> TGFNLSIDTVEGNPGSSVVVPVKLSGISKNGISTADFTVTYDATKLEYISGDAGSIVTNPGVNFGI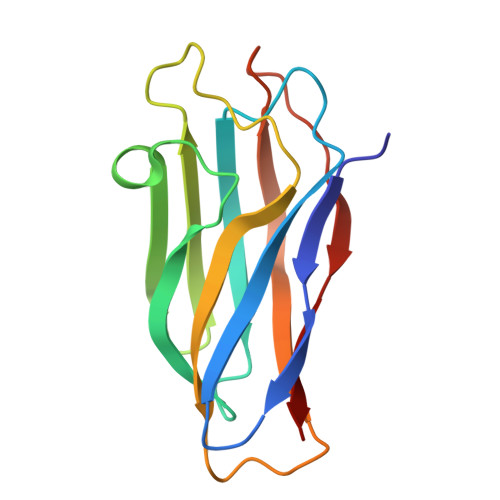NKESDGKLKVLFLDYTMSTGYISTDGVFANLNFNIKSSAAIGSKAEVSISGTPTFGDSTLTPVVAKVTNGAVNLE>[4x]MSEVEFSHEYWMRHALALAKRARDEREVPVGAVLVLNNRVIGEGWNRGIGLHDPTAHA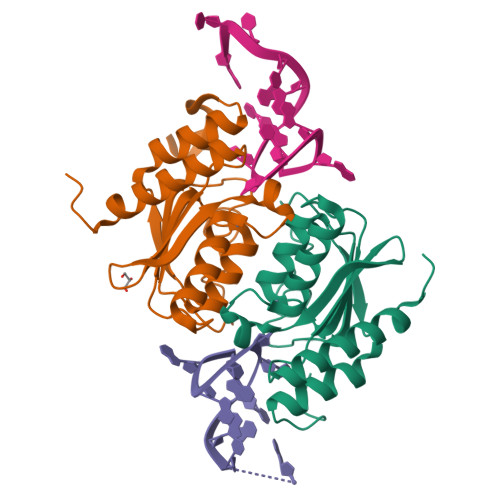EIMALRQGGLVMQNYRLYDATLYTTFEPCVMCAGAMIHSRIGRVVFGVRNAKTGAAGSLMDVLHHPGMNHRVEITEGILADECEALLCRFFRMPRRVFNAQKKAQSSTD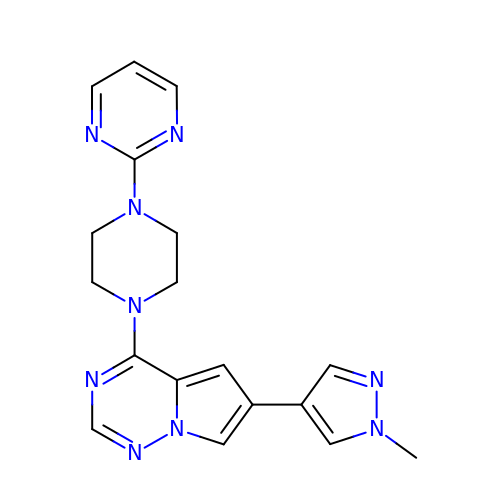6-(1-methylpyrazol-4-yl)-4-(4-pyrimidin-2-ylpiperazin-1-yl)pyrrolo[2,1-f][1,2,4]triazine | C18 H19 N9 | HKKJTAWWASVXFI-UHFFFAOYSA-N UDP-N-acetylglucosamine acyltransferase (LpxA) catalyzes the first step of lipid A biosynthesis. LpxA catalyzes the transfer of an R-3-hydroxymyristoyl chain from ACP to the 3-OH glucosamine group of UDP-GlcNAc. The crystal structure of LpxA reveals a homotrimer that possesses a left-handed parallel β-helix. The active site is located in a deep cleft between adjacent subunits where there are multiple conserved histidines and other basic residues.

Here we report the successful crystallization of E. coli LpxA complexed with peptide CR20 (WMLDPIAGKWSR) at a resolution of 1.60 Å. Peptide CR20 is a potent inhibitor of E. coli LpxA with an IC50 of ~50 nM. There is a single LpxA molecule in the asymmetric unit, and three asymmetric units associate around a crystallographic three-fold axis to form the homotrimer of LpxA. LpxA-bound peptide CR20 is folded into a β-hairpin conformation. The hairpin inserts into the active site of LpxA and the N and C termini of the peptide is solvent exposed. Peptide CR20 does not disrupt any contacts between the individual monomers of LpxA, but instead forms a bridge between the adjacent subunits. Residues of LpxA involved in direct hydrogen bonds with the peptide are Q161 (backbone N) and R258 from one protomer and G155, G173, and M170 from the adjacent protomer. Residues that interact with peptide CR20 via water-mediated interactions are R204, R205, N198, and Q161 (side chain) from the blue chain and H160 from the pink chain. The most efficacious peptide CR20 binds in a region that would mainly occlude the binding site of acyl-ACP.

> WMLDPIAGKWSR;> MIDKSAFVHPTAIVEEGASIGANAHIGPFCIVGPHVEIGEGTVLKSHVVVNGHTKIGRDNEIYQFASIGEVNQDLKYAGEPTRVEIGDRNRIRESVTIHRGTVQGGGLTKVGSDNLLMINAHIAHDCTVGNRCILANNATLAGHVSVDDFAIIGGMTAVHQFCIIGAHVMVGGCSGVAQDVPPYVIAQGNHATPFGVNIEGLKRRGFSREAITAIRNAYKLIYRSGKTLDEVKPEIAELAETYPEVKAFTDFFARSTRGLIR> MQQAPDPAIRAALQSQPSGIASDDWEAAMQRIMALTTRNPESFRQQPQANRLSAILEAVVPSRTNPTHEKVLAIVNALAENKAIRPDEAGLVYNALLERVGRYNSTNVQSNLDRLVTDVREAVAQRERFKNEGLGSLVALNAFLATQPANVPRGQDD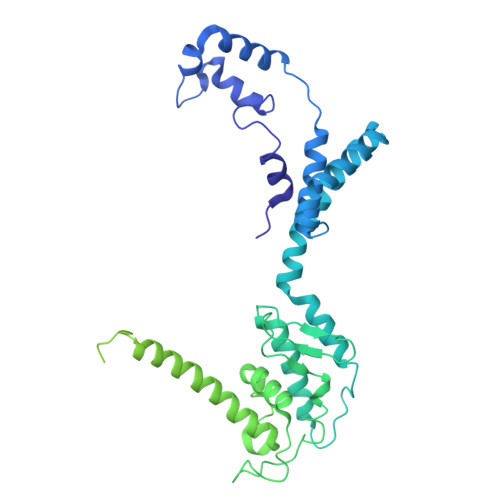YTNFISALRLMVTEVPQSEVYQSGPDYFFQTSRQGLQTVNLSQAFKNLRGLWGVQAPVGDRSTVSSLLTPNSRLLLLLIAPFTDSGSVNRNSYLGHLLTLYREAIGQAQVDEQTFQEITSVSRALGQNDTDSLRATLNFLLTNRQQKIPAQYALSAEEERILRYVQQSVGLFLMQEGATPSAALDMTARNMEPSMYAANRPFINKLMDYLHRAAVMNTDYFTNAILNPHWLPPPGFYTGEYDMPDPNDGFLWDDVDSVVFSPTFQKRQEAPPSEGAVGRSPFPSLGSLHSLPGSVNSGRVSRPRLLGEDEYLNDSLLQPPRAKNAMANNGIESLVDKLNRWKTYAQDHRDAPAPRRQRHDRQRGLVWDDEDSADDSSVLDLGGSGGVNPFAHLQPKLGRRMF>GSHMASPSNTDYPGPHSFDVSFQQSSTAKSATWTYSTELKKLYCQIAKTCPIQIKVMTPPPQGAVIRAMPVYKKAEHVTEVVKRCPNHELSREFNEGQIAPPSHLIRVEGNSHAQYVEDPITGRQSVLVPYEPPQVGTEFTTVLYNFMCNSSCVGGMNRRPILIIVTLETRDGQVLGRRCFEARI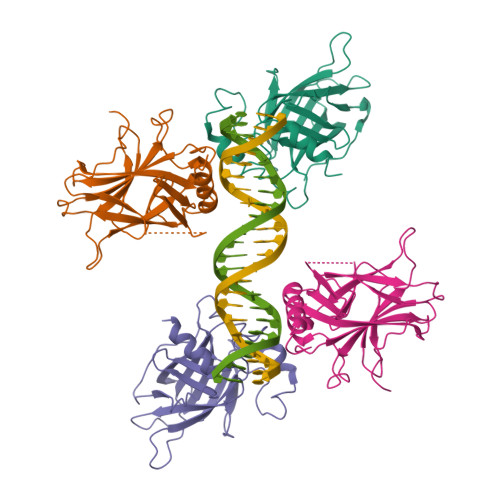CACPGRDRKADEDSIRKQ[4x]> GAACGACAGAGA;> CGCCGACTC;> TCTGCG;> TCGAGTCGCTGTCGT

In this work, we exhaustively probe the ability of all 36 immobile HJ sequences to form DNA crystals in two different designed systems. Three separate self-assembling DNA crystal systems are described in this report: the “4 × 5” and “4 × 6” designs (collectively referred to as the 4 × N systems), and a third construct with a “scrambled” sequence variant of the 4 × 6 lattices. Self-assembly was mediated by three constituent oligonucleotides: (S1) containing four sequence repeats of either 5 or 6 bases; (S2) composed of 21 bases containing complementary regions to both (S1); and (S3) which forms the second junction crossover. The HJ serves as the fundamental component at the core of each unit, and the ultimate assembly of the full lattice is facilitated by the complementary 2-base sticky ends that tail each duplex.

Because the 4 × 6 system yielded R3 symmetry in 5 of 17 junctions, we considered whether the downstream sequences adjacent to the junction could play a role in crystallization efficiency, junction angle, and symmetry preference, or if the HJ alone was the singular determinant. To investigate this possibility, we designed “scrambled” sequences with targeted base substitutions, while maintaining GC content, along each “stem”. Contrary to the buffer preference observed with the native P32 crystals, the scrambled systems exhibited an exclusive preference towards low salt buffers, much like the native R3 crystals. Remarkably, only J1 and J2 retained the P32 symmetry, with all others yielding an R3 lattice. There appeared to be only a marginal difference in the average cell lengths in the R3 scramble crystals (a = b = 113.04 c = 51.10) relative to the native 4 × 6 sequences: the a, b axis trended ~2 Å shorter and c ~1.3 Å longer, whereas in the J1 and J2 cases, the crystals were in good agreement with the original 4 × 6 motif. The average angles of the R3 and P32 crystals were 61.00° (σ = 1.21) and 58.05° (σ = 1.39), respectively. Further, we observed modest improvements in resolution, reaching as high as 2.7 Å in J36. Notably, all junctions preventing crystallization compared to its original counterpart remained fatal and all relative cavity dimensions and volumes remained unperturbed. However, in the majority of the crystal structures reported here, the cacodylate anion indeed fits best into the electron density map of our X-ray structures, due to the presence of sodium cacodylate in the crystallization solution. A complete description of the comprehensive, experimental evidence for this arsenic has been described in our previous work. This seemingly counterintuitive result can be rationalized in several ways: First, the cacodylate could be stabilized at this site by hydrogen bonding and interactions with the solvent, both of which are known to provide stabilization for anionic binding even at regions with negative surface potentials.>[2x]MH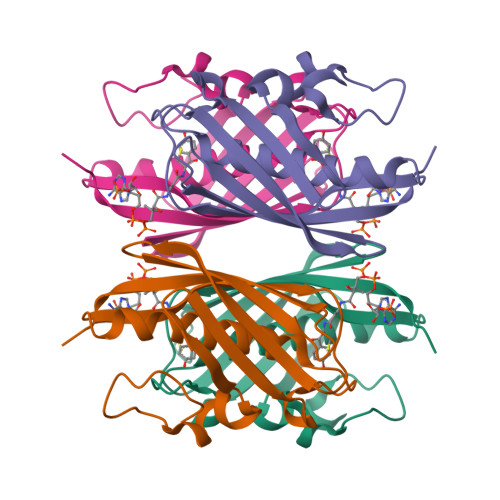RTSNGSHATGGNLPDVASHYPVAYEQTLDGTVGFVIDEMTPERATASVEVTDTLRARWGLVHGGAYCALAEMLATEATVAVVHEKGMMAVGQSNHTSFFRPVKEGHVRAEAVRIHAGSTTWFWDVSLRDDAGRLCAVSSMSIAVRPRRD>[2x]MKRQWALEDFEIGRPLGKGKFGNVYLAREKQSKFILALKVLFKAQLEKAGVEHQLRREVEIQSHLRHPNILRLY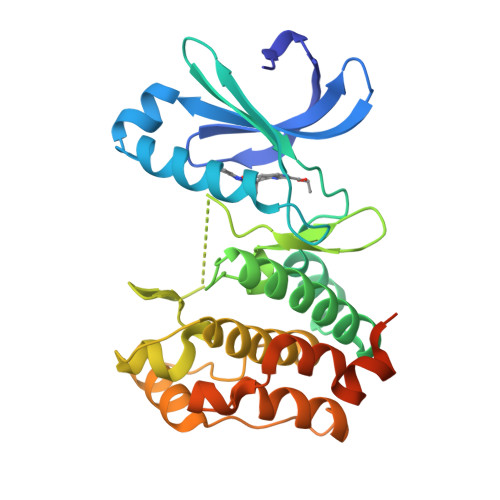GYFHDATRVYLILEYAPLGTVYRELQKLSKFDEQRTATYITELANALSYCHSKRVIHRDIKPENLLLGSAGELKIADFGWSVHAPSSRRTTLCGTLDYLPPEMIEGRMHDEKVDLWSLGVLCYEFLVGKPPFEANTYQETYKRISRVEFTFPDFVTEGARDLISRLLKHNPSQRPMLREVLEHPWITANSSKPSNCQNKESAAAALEHHHHHH(5Z)-5-(quinolin-6-ylmethylidene)-2-[(thiophen-2-ylmethyl)amino]-1,3-thiazol-4(5H)-one | C18 H13 N3 O S2 | 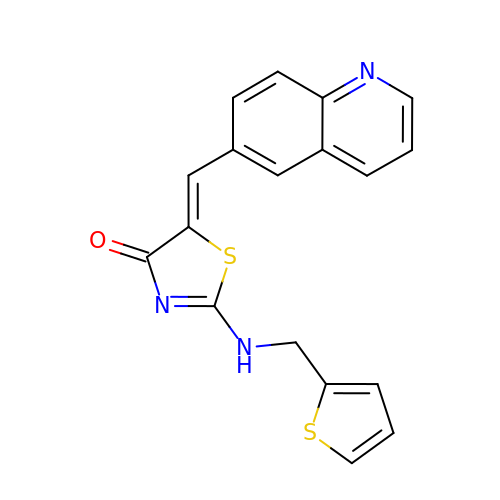XOLMRFUGOINFDQ-YBEGLDIGSA-N2,2,2-TRIFLUORO-1-{5-[(3-PHENYL-5,6-DIHYDROIMIDAZO[1,2-A]PYRAZIN-7(8H)-YL)CARBONYL]THIOPHEN-2-YL}ETHANE-1,1-DIOL 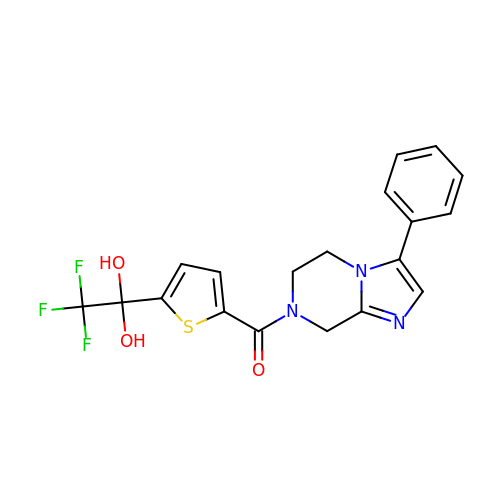| C19 H16 F3 N3 O3 S | OFBFUNBBOQCNFX-UHFFFAOYSA-N>MGSSHHHHHHGTAENLYFQGERKYSTFYEQRATLFEELPVTSKDIIFLGNSITNGCEWAELFQNKNVKNRGISGDICMGVYDRLDPIVKGKPAKIFLLIGINDVSRGTSADKIISEISMIVRKIKQESPKTKLYLQSVLPVNDCYGMFNGHTSRWQVVKQINDLLEPLAVKEGVAYIDLYSHFVEKETGKMNPVYTNDGLHLLGKGYLLWRDIVKPYVDQK[4x]

Here, the crystal structure of a 9-O-SAE from Phocaeicola vulgatus (PvSAE) is reported. Structural characterization revealed PvSAE to be a dimer with an SGNH fold, named after the conserved sequence motif of this family, and a Ser–His–Asp catalytic triad. Biochemical assays also show that PvSAE deacetylates both mucin and the acetylated chromophore para-nitrophenyl acetate. Therefore, bacteria employ esterases to make acetylated sialic acid more accessible for cleavage by sialidases.

A crystal from the Apo I condition diffracted to a resolution of 1.44 Å and had P1211 symmetry, while a crystal from the Apo II condition diffracted to 2.06 Å resolution and had P61 symmetry. The most significant difference between the Apo I and Apo II structures was the positioning of the most N-terminal residues (residues 24–27) of the first α-helix. In the Apo I structure residues 24–27 of one of the protomers in the homodimer are no longer part of this α-helix structure, but instead form a loop projecting out of the active site. This conformational change is supported by a hydrogen bond between the hydroxyl of Tyr25 and the carboxylic acid of Asp83 from the neighbouring protomer. The result of this change in conformation is that one active site is more accessible and has an ‘open’ conformation, while the other is still ‘blocked’ by the N-terminal α-helix. We suspect that this conformational change may be important for the accommodation of large, complex glycans that contain acetylated sialic acid. The high resolution of the Apo I structure allowed the identification of a malonate molecule in the active site of PvSAE. Malonate is positioned such that a carboxylate functional group is within hydrogen-bonding distance of the oxyanion-hole residues Asn103 and Gly75. As the most N-terminal α-helix of the Apo I structure has different conformations, the two active sites accommodate the modelled 9-O-acetylsialic acid in a different conformation. In the ‘open’ active site, the 9-O-acetylsialic acid is positioned such that the 2-position projects towards the bulk solvent, indicating that this site could accommodate larger glycans.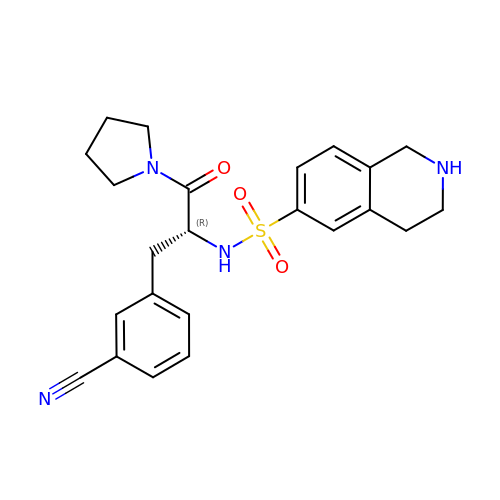(R)-(3-(3-cyanophenyl)-1-oxo-1-(pyrrolidin-1-yl)propan-2-yl)-1,2,3,4-tetrahydroisoquinoline-6-sulfonamide | C23 H26 N4 O3 S | WWKTZMSNGFQJAG-JOCHJYFZSA-N ORF3a is a transmembrane protein capable of forming homodimers and potentially homotetramers. The TRAF proteins participate in multiple NF-κB signaling pathways, functioning as adaptor proteins and E3 ubiquitin ligases. They form trimers and interact with receptor intracellular domains and other proteins through their C-terminal TRAF-C domains. Since the putative TRAF-binding sequence in ORF3a is conserved between SARS-CoV (PLQAS) and SARS-CoV-2 (PIQAS), and generally conforms to the TRAF-binding consensus sequences, we hypothesized that SARS-CoV-2 ORF3a might also bind to TRAFs and thereby induce NF-κB activation.

To investigate whether the SARS-CoV-2 ORF3a N-terminal region containing the PIQAS sequence is capable of binding to TRAF molecules, we crystallized the TRAF2 TRAF-C domain and the TRAF3 TRAF-C domain in complex with a 16-amino acid peptide from the N-terminal region of ORF3a (residues 30–45). The crystallographic asymmetric unit in the TRAF2 crystal lattice contains three TRAF-C molecules forming a trimer, while the asymmetric unit in the TRAF3 crystal lattice contains six TRAF-C molecules forming two trimers. We observed density for five residues (PIQAS) of the ORF3a peptide, which binds at a solvent-facing groove in the globular region of the TRAF-C domain. The TRAF-C binding sites are not fully occupied—in our model, each TRAF trimer has either one or two peptides bound, which is similar to previously reported TRAF:peptide complex structures. We also co-crystallized TRAF2 TRAF-C with an ORF3a peptide in which the isoleucine was replaced with selenomethionine and collected anomalous diffraction data. The anomalous difference density map at 4 sigma clearly shows the position of the heavy selenium atom, which further confirms the position of the PIQAS peptide bound at the TRAF-C domain groove. The ORF3a peptide forms several main chain and side chain hydrogen bonds with the surrounding residues from TRAF2 or TRAF3. Of note, the side chain from Q38 in the peptide forms multiple hydrogen bonds with two serine residues in the TRAF-C domain. The binding affinities between the PIQAS peptide and SUMO-TRAF-C proteins were in the range of 150–200 μM (192.5 μM for TRAF2 and 171.6 μM for TRAF3). Crystal structures revealed that a PIQAS-containing peptide can bind to TRAF2 or TRAF3 at the previously identified peptide-binding surface in the TRAF-C domain.

>[6x]SEALSSKVQQLERSIGLKDLAMADLEQKVLEMEASTYDGVFIWKISDFARKRQEAVAGRIPAIFSPAFYTSRYGYKMCLRIYLNGDGTGRGTHLSLFFVVMKGPNDALLRWPFNQKVTLMLLDQNNREHVIDAFRPDVTSSSFQRPVNDMNIASGCPLFCPVSKMEAKNSYVRDDAIFIKAIVDLTGL;>[3x]PIQAS> MTHRFPRSRTALAVALMAGFAMSAQARVFRSADVHGDSFPTNMAVKFMGDELSKLTGGKDSIKVFGNSALGSEKDTVDQVRIGAIDMARVNGASFNEIVPESLIPSFPFLFRDVDHFRKAMYGPAGQKILDAFAAKGMIALTFYESGARSIYAKRPVRTPADMKGLKVRVQPSDLMVDEIRAMGGTPTPMPFAEVYTGLKTGLVDAAENNLPSYEETKHF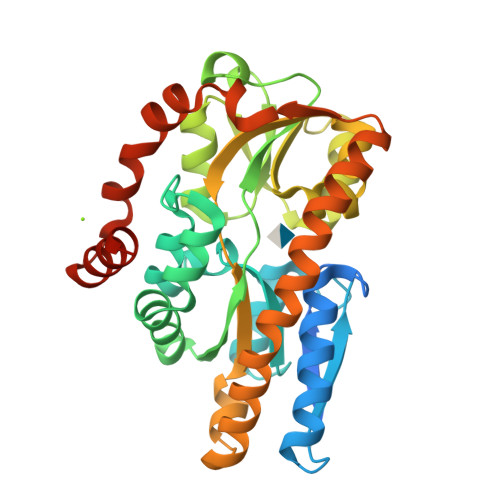EVAPDYSETQHAMTPEVLVFSKKIWDTLSPQEQAAIRKAAADSVPYYQKLWTAREASAQQAVTKGGANILPAAQVDRAAFVKAMQPLWTKYEKTPQMKQIVDEIEATKAENLYFQ> MGHHHHHHSIETDRVSKEFIEFLKTFHKTGQEIYKQTKLFLEGMHYKRDLSIEEQSECAQDFYHNVAERMQTRGKVPPERVEKIMDQIEKYIMTRLYKYVFCPETTDDEKKDLAIQKRIRALRWVTPQMLCVPVNEDIPEVSDMVVKAITDIIEMDSKRVPRDKLACITKCSKHIFNAIKITKNEPASADDFLPTLIYIVLKGNPPRLQSNIQYITRFCNPSRLMTGEDGYYFTNLCCAVAFIEKLDAQSLNLSQEDFDRYMSQMYKNLDLLSQLNERQERIMNEAKKLEKDLIDWTDGIAREVQDIVEK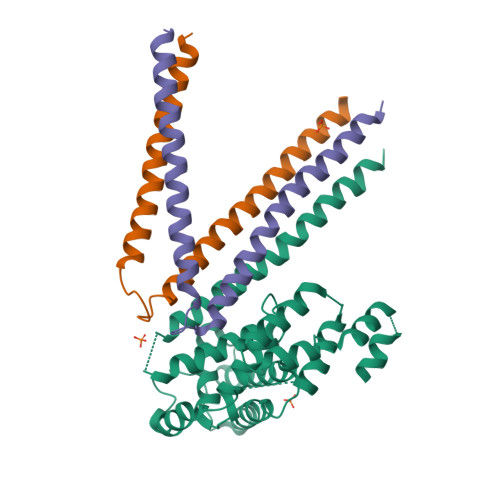;>METRDQVKKLQLMLRQANDQLEKTMKDKQELEDFIKQSSEDSSHQISALVLRAQASEILLEELQQGLSQAKRDVQEQMAVLMQSREQVSEEL[2x]6-(2-fluoranylpyridin-4-yl)-~{N}-[(1~{R})-1-(3-methoxyphenyl)ethyl]pyridine-3-carboxamide 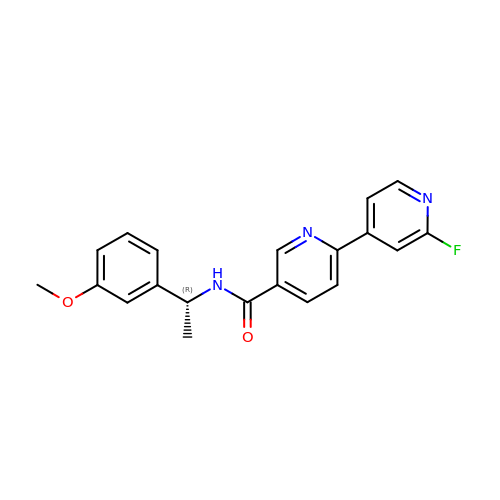| C20 H18 F N3 O2 | HZBPSQIDFQPUKG-CYBMUJFWSA-N>MSKNKVVIIGAGFAGLVAARELQTAGIEYEILEAKDRIGGRAWTEERMGRPLELGATWVHWFQAHTWTEIMRYGQRTEITASPSGNDAHWVTDGKVVKGTEDDLDEKLTAAMGVTYEGSEEYFPNPHDPLWVLSDDFDGPAEVRERFLSDDQTNAIDLVKEAGFDQETIDLVDAFWCAGYIGDPYTGSALMAKQWGALSDNRYRVMEDITLKWKLNNGMRSLYDGIAGDLNTDIRLNTPVAKVEHHDNGATVTTESGEVIEASAVICTVPVGALSNIEFSPALPDAVQSVIDDKWNSQGAKIWIKIKGHHRFLGYAPKPAKMSVVRSEYFMDDDTTILVGFGYDNTNIDLNSIEDAQAVINQWRDDLEVVDTTGHNWVADKWAGQAWGTLRKGQFTQGWSLFDDIDSQLFFAGSDYAYGWRGVSVDGALEKGMTTARQVINSMRETKE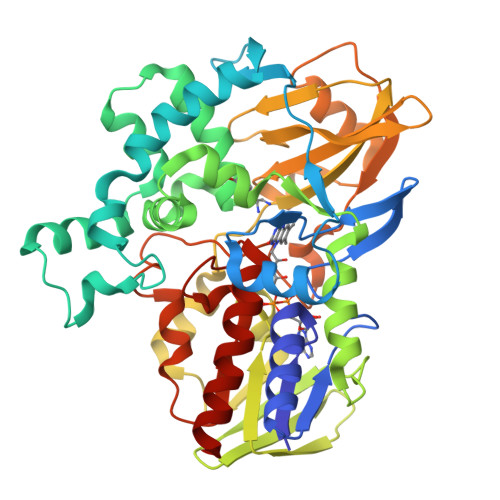Q[2x]hexyl (5S,6R,8R)-6-hydroxy-5-methyl-13-oxo-5,6,7,8-tetrahydro-13H-5,8-epoxy-4b,8a,14-triazadibenzo[b,h]cycloocta[1,2,3,4-jkl]cyclopenta[e]-as-indacene-6-carboxylate | C32 H29 N3 O5 | 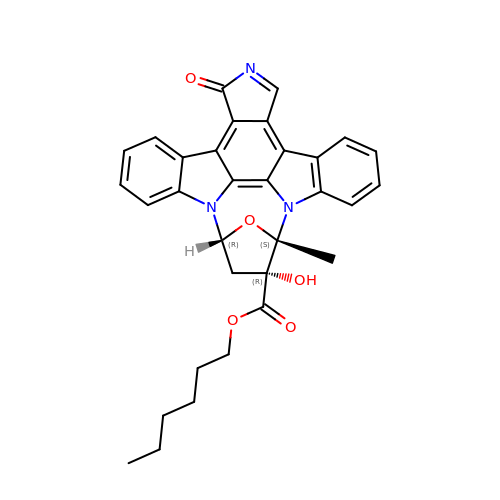ZDVKBGNYCWCWDZ-MWOZDUBJSA-N> MNELSKKYLAKVKERHELKEFNNSISAQDNYAKWTKNNRKLDSLDKEINNLKDEIQSENH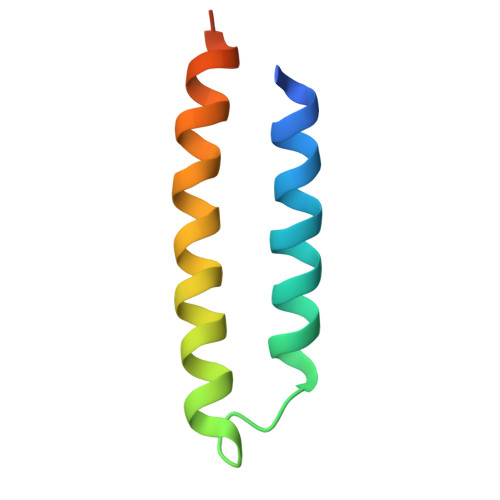HHHHH>[8x]MNHKVHHHHHHMELGTLEGSENLYFQGAMARGVNKVI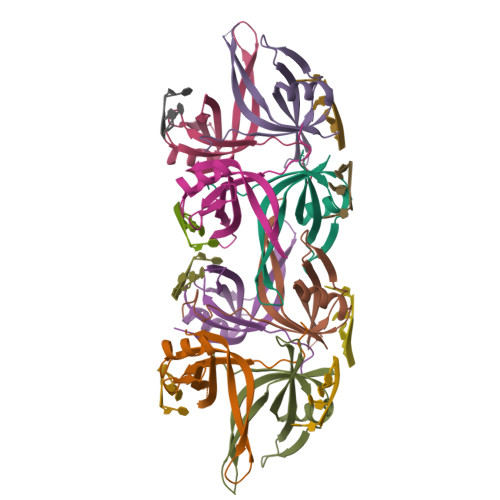LIGNLGDDPELRYTGSGTAVCNMSLATNETYTDSDGNEVQNTEWHDVVAWGRLGEICNEYLDKGSQVYFEGKLQTRSWEDRDNNTRYSTEVKAQEMMFLDSNRQGGADMDGFDQTRGDESLDQTRQEQPAGSSGPQPGQQASSGGEDEDTFEPDDDLPF>EVCNDEVDLYLLMDGSGSIRRHNWVNHAVPLAMKLIQQLNLNDNAIHLYASVFSNNAREIIRLHSDASKNKEKALIIIKSLLSTNLPYGKTSLTDALLQVRKHLNDRINRENANQLVVILTDGIPDSIQDSLKESRKLSDRGVKIAVFGIGQGINVAFNRFLVGCHPSDGKCNLYADSAW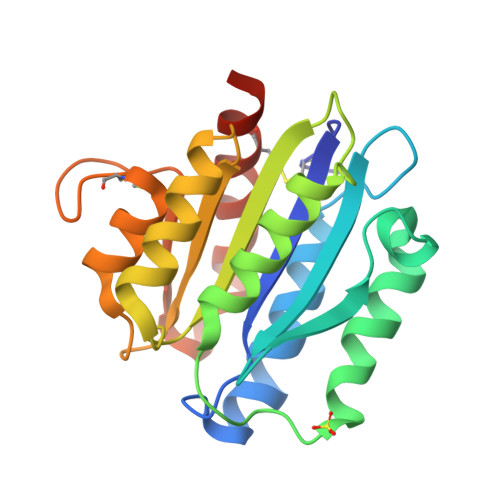ENVKNVIGPFMKAVCVEVEKHHHHHHA[2x]>[2x]MNKQKISPAEVAKHNKPDDCWVVINGYVYDLTRFLPNHPGGQDVIKFNAGKDVT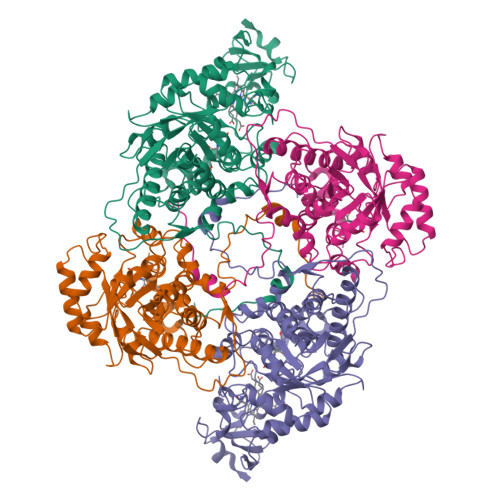AIFEPLHAPNVIDKYIAPEKKLGPLQGSMPPELVCPPYAPGETKEDIARKEQLKSLLPPLDNIINLYDFEYLASQTLTKQAWAYYSSGANDEVTHRENHNAYHRIFFKPKILVDVRKVDISTDMLGSHVDVPFYVSATALCKLGNPLEGEKDVARGCGQGVTKVPQMISTLASCSPEEIIEAAPSDKQIQWYQLYVNSDRKITDDLVKNVEKLGVKALFVTVDAPSLGQREKDMKLKFSNTKAGPKAMKKTNVEESQGASRALSKFIDPSLTWKDIEELKKKTKLPIVIKGVQRTEDVIKAAEIGVSGVVLSNHGGRQLDFSRAPIEVLAETMPILEQRNLKDKLEVFVDGGVRRGTDVLKALCLGAKGVGLGRPFLYANSCYGRNGVEKAIEILRDEIEMSMRLLGVTSIAELKPDLLDLSTLKARTVGVPNDVLYNEVYEGPTLTEFEDA>[2x]RRRTCLPAPCPSSSNISLWNILRNNIGKDLSKVAMPVELNEPLNTLQRLCEELEYSELLDKAAQIPSPIERMVYVAAFAISAYASSYY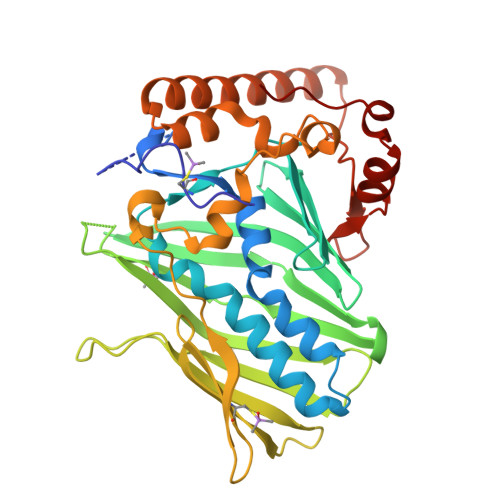RAGSKPFNPVLGETYERIREDKGFQFFSEQVSHHPPISACHAESRNFVFWQDVRWKNKFWGKSMEIVPIGTTHVTLPVFGDHFEWNKVTSCIHNILSGQRWIEHYGEIVIKNLHDDSCYCKVNFIKAKYWSTNAHEIEGTVFDRSGKAVHRLFGKWHESIYCGGGSSSACVWRANPMPKGYEQYYSFTQFALELNEMDPSSKSLLPPTDTRFRPDQRFLEEGNLEEAEIQKQRIEQLQRERRRVLEENHVEHQPRFFRKSDDDSWVSNGTYLELRKDLGFSKLDHPVLW>[2x]TAGGGTTA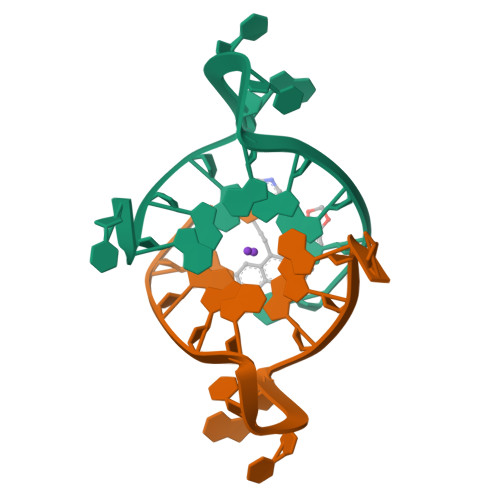GGGT>[6x]VPRPPAPLFRDPIYDGAADPTIIYNHLEKSWWILYTNRRANQKLPGKAFMHGTDIGIAESKDGGRTWFYRGTIELQYGRGRNTFWAPEVIFYEGEYHMYVSFVPGVPQDWNAERYILYYKSKNLWDWEFVCKLELSSNKVIDACVFQMPDGTFRMWYKDEADHSYIYAAESNNLKDWKILGPALTDRPQEGPNVFWWKSKYWMITDPWCGLGVYSSEDATAWHRHENILDRPGKREDDGQIGHHADVLVIDDETAYIFYFTHPEGMEGTEEFWKDSKYWRTSLQVAKLEYVDGKVVCDRDKEFDFYLPDLFAHHHHHH

Functional, biochemical, and preliminary structural properties are reported for three glycoside hydrolases of the recently described glycoside hydrolase (GH) family 159. Even though the thermophilic enzymes investigated—Cs_Gaf159A, Ch_Gaf159A, and Ck_Gaf159A—cleaved pNP-α-l-arabinofuranoside, they were only weakly active on arabinogalactan, and they did not cleave arabinose from arabinan, arabinoxylan, or gum arabic. However, the enzymes were able to hydrolyze the α-1,3-linkage in different arabinoxylan-derived oligosaccharides (AXOS) with arabinosylated xylose at the non-reducing end (A3X, A2,3XX), suggesting their role in the intracellular hydrolysis of oligosaccharides. Like some other glycoside hydrolases, Cs_Gaf159A, Ch_Gaf159A, and Ck_Gaf159A are activated by divalent metal ions.

Crystallization and structural analysis of the apo form of one of the Caldicellulosiruptor enzymes, Ch_Gaf159A, enabled the elucidation of the first 3D structure of a GH159 member. However, Ch_Gaf159A is substantially smaller than its homologues, consisting of only a five-bladed β-propeller domain. Each blade is composed of four mainly antiparallel beta-strands. The stable monomeric state of Ch_Gaf159A was confirmed by means of polymerization-induced self-assembly (PISA) calculations and size-exclusion chromatography. The fold of Ch_Gaf159A displays striking similarities to that of glycoside hydrolase family 43. The positions of E190, D142, and D19 in Ch_Gaf159A exactly matched E186, proposed to be the nucleophilic catalytic base, D127, and D14 in XynB. E190 in Ch_Gaf159A is suggested as being catalytically important given its proximity to the glycosidic O and its description as a catalytic base in XynB. The surface representation showed two electro negative pockets, one of them capable of incorporating the X2 ligand. This substrate pocket structurally explains why Ch_Gaf159A acts as an exo-arabinofuranosidase, or -galactofuranosidase. The complete loss of activity of the Ch_Gaf159A mutants D19A, D142A and E190A, which was tested with pNPA, AXOS and arabinogalactan, confirmed this prediction.2-(4-bromanyl-3-oxidanyl-phenyl)-1-[(1R)-2-[2-(2-tert-butylphenoxy)ethanoylamino]-1-(3,4-dimethoxyphenyl)ethyl]-N-methyl-benzimidazole-5-carboxamide 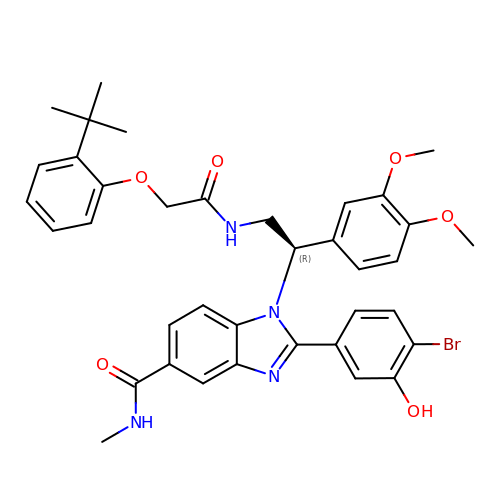| C37 H39 Br N4 O6 | NVXVCMOQLYUYSD-LJAQVGFWSA-N>PSVYDAAAQLTADVKKDLRDSWKVIGSDKKGNGVAMMTTLFADNQETIGYFKRLGDVSQGMANDKLRGHSITLMYALQNFIDQLDNPDDLVCVVEKFAVNHITRKISAAEFGKINGP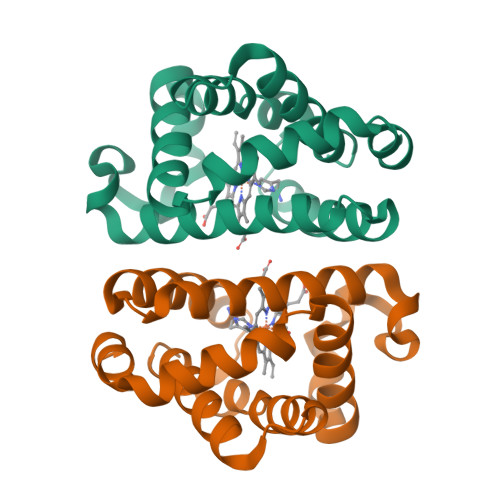IKKVLASKNFGDKYANAWAKLVAVVQAAL[2x]>[2x]MVVIGEKFPEVEVKTTHGVIKLPDYFTKQGKWFILFSHPADFTPVCTTEFYGMQKRVEEFRKLGVEPIGLSVDQVFSHIKWIEWIKDNLSVEIDFPVIADDRGELAE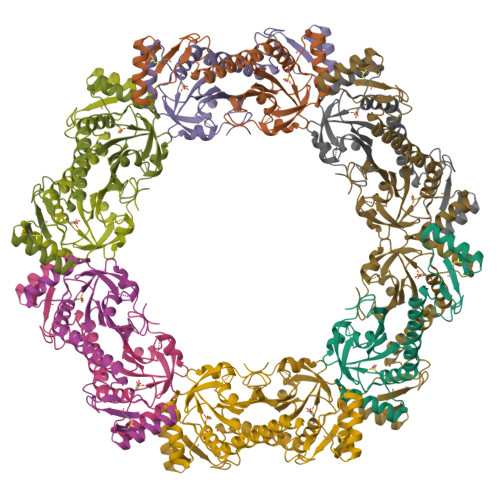KLGMIPSGATITARAVFVVDDKGIIRAIVYYPAEVGRDWDEILRLVKALKISTEKGVALPHKWPNNELIGDKVIVPPASTIEEKKQREEAKAKGEIECYDWWFCYKKLE>MLDPRLSVAPMVDRTDRHFRFLVRQVSLGVRLYTEMTVDQAVLRGNRERLLAFRPEEHPIALQLAGSDPKSLAEAARIGEAFGYDEINLNLGCPSEKAQEGGYGACLLLDLARVREILKAMGEAVRVPVTVKMRLGLEGKETYRGLAQSVEAMAEAGVKVFVVHARSALLALSTKANREIPPLRHDWVHRLKGDFPQLTFVTNGGIRSLEEALFHLKRVDGVMLGRAVYEDPFVLEEADRRVFGLPRRPSRLEVARRMRAYLEEEVLKGTPPWAVLRHML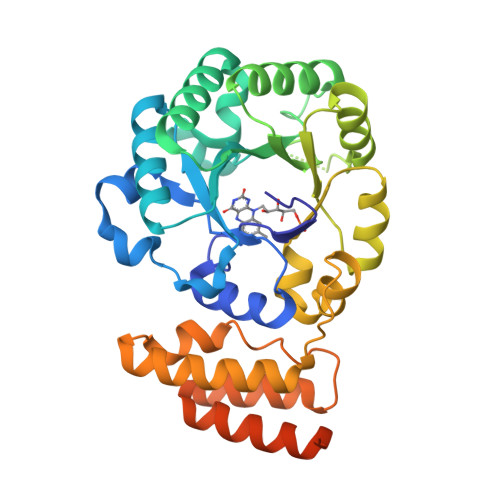NLFRGRPKGRLWRRLLSEGRSLQALDRALRLMEEEVGEEGEKEKPGPRGQREAAPGPAREGVLEHHHHHH[2x]> GPMTVFRQENVDDYYDTGEELGSGQFAVVKKCREKSTGLQYAAKFIKKRRTKSSRRGVSREDIEREVSILKEIQHPNVITLHEVYENKTDVILILELVAGGELFDFLAEKESLTEEEATEFLKQILNGVYYLHSLQIAHFDLKPENIMLLDRNVPKPRIKIIDFGLAHKIDFGNEFKNIFGTPEFVAPEIVNYEPLGLEADMWSIGVITYILLSGASPFLGDTKQETLANVSAVNYEFEDEYFSNTSALAKDFIRRLLVKDPK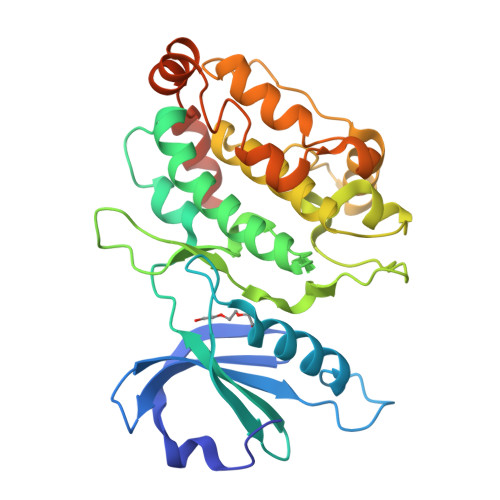KRMTIQDSLQHPWIKPKDTQQALSRKACAVNMEKFKKFAARKKWKQSVRLISLCQRLSRS(~{E})-~{N}-[4-(4-azanyl-1-propan-2-yl-pyrazolo[3,4-d]pyrimidin-3-yl)phenyl]-4-[4-fluoranyl-3-(trifluoromethyl)phenyl]-4-oxidanylidene-but-2-enamide | C25 H20 F4 N6 O2 | 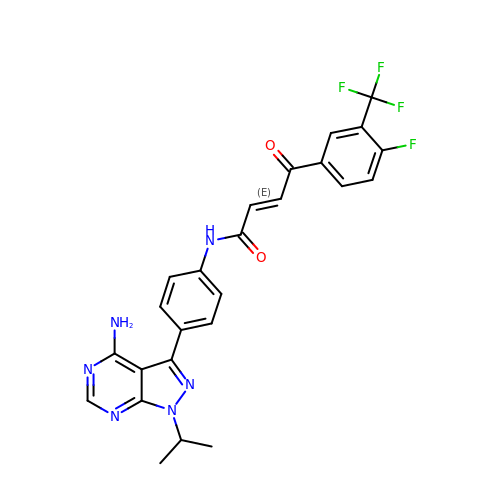UNZLHTLRBOOXGC-MDZDMXLPSA-N>MDERDALRISREIAGEVRKAIASMPLREAVKDVGMGKDGTPTKAADRVAEDAALEILRKERVTVVTEESGVLGEGDVFVALDPLDGTFNATRGIPVYSVSLCFSYSDKLKDAFFGYVYNLATGDEYYADSSGAYRNGERIEVSDAEELYCNAIIYYPDRKFPFKRMRIFGSAATELCFFADGSFDCFLDIRPGKMLRIYDAAAGVFIAEKAGGKVTELDGESLG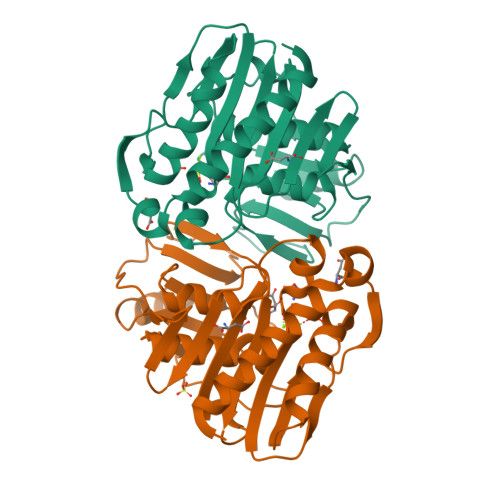NKKFDMQERLNIVAANEKLHPKLLELIK[2x]> GHMSGRGKKPTRTLVMTSMPSEKQNVVIQVVDKLKGFSIAPDVCETTTHVLSGKPLRTLNVLLGIARGCWVLSYDWVLWSLELGHWISEEPFELSHHFP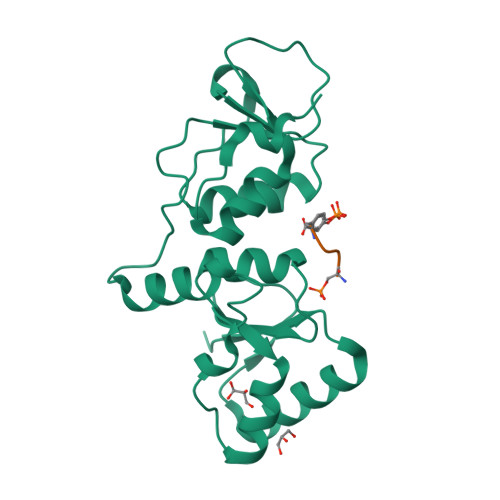AAPLCRSECHLSAGPYRGTLFADQPVMFVSPASSPPVAKLCELVHLCGGRVSQVPRQASIVIGPYSGKKKATVKYLSEKWVLDSITQHKVCAPENYLLSQ;> SQEY>[2x]MNVTVSIPTILRPH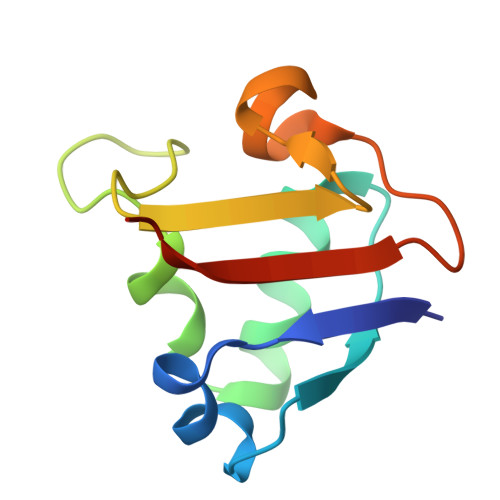TGGQKSVSASGDTLGAVISDLEANYSGISERLMDPSSPGKLHRFVNIYVNDEDVRFSGGLATAIADGDSVTILPAVAGG> ALVKE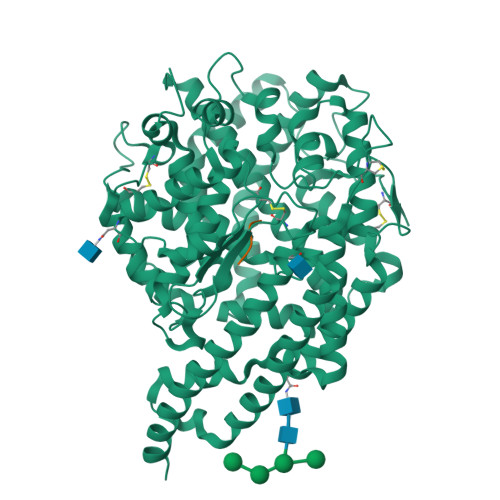EIQAKEYLENLNKELAKRTNVETEAAWAYGSNITDENEKKKNEISAELAKFMKEVASDTTKFQWRSYQSEDLKRQFKALTKLGYAALPEDDYAELLDTLSAMESNFAKVKVCDYKDSTKCDLALDPEIEEVISKSRDHEELAYYWREFYDKAGTAVRSQFERYVELNTKAAKLNNFTSGAEAWLDEYEDDTFEQQLEDIFADIRPLYQQIHGYVRFRLRKHYGDAVVSETGPIPMHLLGNMWAQQWSEIADIVSPFPEKPLVDVSAEMEKQGYTPLKMFQMGDDFFTSMNLTKLPQDFWDKSIIEKPTDGRDLVCHASAWDFYLTDDVRIKQCTRVTQDQLFTVHHELGHIQYFLQYQHQPFVYRTGANPGFHEAVGDVLSLSVSTPKHLEKIGLLKDYVRDDEARINQLFLTALDKIVFLPFAFTMDKYRWSLFRGEVDKANWNCAFWKLRDEYSGIEPPVVRSEKDFDAPAKYHISADVEYLRYLVSFIIQFQFYKSACIKAGQYDPDNVELPLDNCDIYGSAAAGAAFHNMLSMGASKPWPDALEAFNGERIMSGKAIAEYFEPLRVWLEAENIKNNVHIGWTTSNKCVS;> DRVYIHPF>[2x]KKIFKPEELRQALMPTLEALYRQDPESLPFRQP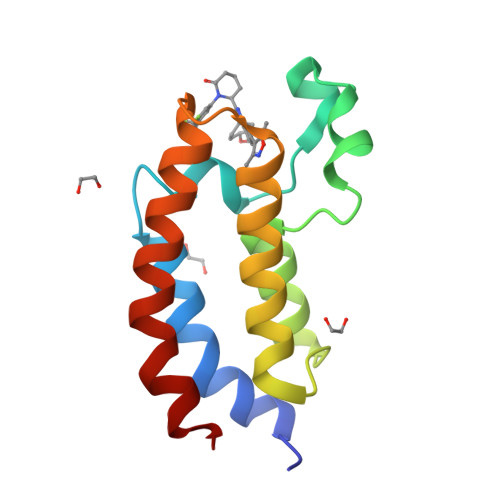VDPQLLGIPDYFDIVKNPMDLSTIKRKLDTGQYQEPWQYVDDVWLMFNNAWLYNRKTSRVYKFCSKLAEVFEQEIDPVMQSLG Human feline leukaemia virus subgroup C receptor-related proteins 1 and 2 (FLVCR1 and FLVCR2) are members of the major facilitator superfamily. Here, we show that FLVCR1 and FLVCR2 facilitate the transport of choline and ethanolamine across the plasma membrane, using a concentration-driven substrate translocation process. Fully conserved tryptophan and tyrosine residues form the binding pocket of both transporters and confer selectivity for choline and ethanolamine through cation–π interactions. Our findings indicate that both FLVCR1 and FLVCR2 operate as uniporters, facilitating downhill ligand transport independent of sodium or pH gradients.

We determined structures of FLVCR1 and FLVCR2 in as-isolated (without exogenous addition of ligands), inward-facing conformations at 2.9 Å resolution. The inward-facing conformations of FLVCR1 and FLVCR2 exhibit a close resemblance to each other, with a root mean square deviation (Cα r.m.s.d.) of 0.993 Å. Both structures feature a wedge-shaped solvent-accessible cavity that is mainly created by the separation of TM4 and TM5 of the N domain from TM10 and TM11 of the C domain. On the level of the outer leaflet, TM1, TM2 and TM5 of the N domain and TM7, TM8 and TM11 of the C domain pack tightly against each other and thus shield the central cavity from the extracellular space. In line with an alternating-access model, the inward-facing conformation of FLVCR2 features a tightly sealed extracellular gate created by interdomain interactions. This is mainly achieved by the juxtaposition of TM1b (N domain) and TM7b (C domain). The interdomain interaction between these two motifs is stabilized by a hydrogen-bonding network consisting of two pseudosymmetry-related asparagine residues N110FLVCR2 and N332FLVCR2 and E343FLVCR2 (TM8) and N239FLVCR2 located on the extracellular loop connecting TM5 and TM6 (EL5–6). Furthermore, we identified a stable interdomain salt bridge between D124FLVCR2 (TM2) and R333FLVCR2 (TM7b), reinforcing the external occlusion. Our cell-based mutagenesis studies show that alanine substitutions at N110FLVCR2, E343FLVCR2, D124FLVCR2 and R333FLVCR2 individually result in a significant decrease of choline uptake and an almost complete perturbation of ethanolamine transport, highlighting a critical role of interdomain interactions on the extracellular surface for FLVCR2 functionality.

> MVNEGPNQEESDDTPVPESALQADPSVSVHPSVSVHPSVSINPSVSVHPSSSAHPSALAQPSGLAHPSSSGPEDLSVIKVSRRRWAVVLVFSCYSMCNSFQWIQYGSINNIFMHFYGVSAFAIDWLSMCYMLTYIPLLLPVAWLLEKFGLRTIALTGSALNCLGAWVKLGSLKPHLFPVTVVGQLICSVAQVFILGMPSRIASVWFGANEVSTACSVAVFGNQLGIAIGFLVPPVLVPNIEDRDELAYHISIMFYIIGGVATLLLILVIIVFKEKPKYPPSRAQSLSYALTSPDASYLGSIARLFKNLNFVLLVITYGLNAGAFYALSTLLNRMVIWHYPGEEVNAGRIGLTIVIAGMLGAVISGIWLDRSKTYKETTLVVYIMTLVGMVVYTFTLNLGHLWVVFITAGTMGFFMTGYLPLGFEFAVELTYPESEGISSGLLNISAQVFGIIFTISQGQIIDNYGTKPGNIFLCVFLTLGAALTAFIKADLRRQKANKETLENKLQEEEEESNTSKVPTAVSEDHLDYKDDDDK> GSHMEGEIDIAKRIEDGINQVQCSVAEYPEAITYLLEQYNRVEAEEARLSDLITGFVDPNAEEDLAPTATHVGSELSQEDLDDDEDEDEEDGDDDSADDDNSIDPELAREKFAELRAQYVVTRDTIKAKGRSHATAQEEILKLSEVFKQFRLVPKQFDYLVNSMRVMMDRVRTQERLIMKLCVEQCKMPKKNFITLFTGNETSDTWFNAAIAMNKPWSEKLHDVSEEVHRALQKLQQIEEETG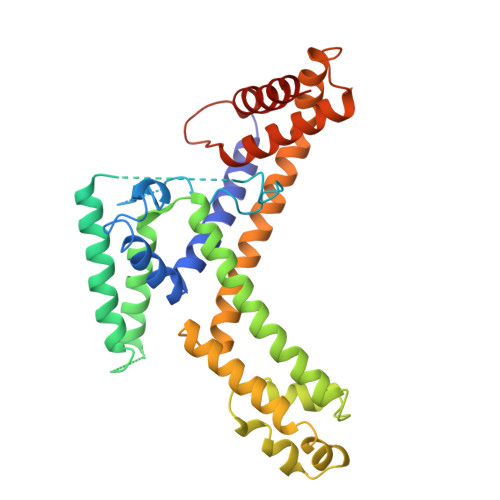LTIEQVKDINRRMSIGEAKARRAKKEMVEANLRLVISIAKKYTNRGLQFLDLIQEGNIGLMKAVDKFEYRRGYKFSTYATWWIRQAITRSIADQAR>[4x]MNNTHGVDSRSDRTSPQDLASAEVAGLPVSALHGTNISTGRGSEADVAEPIQEAVDRKVSELDLAAYDKDDFTQPMIKKIMSRLFSAFDVTHLGYLTPDKVEEVCRYLGRNMSDGDVKAMKAEINAID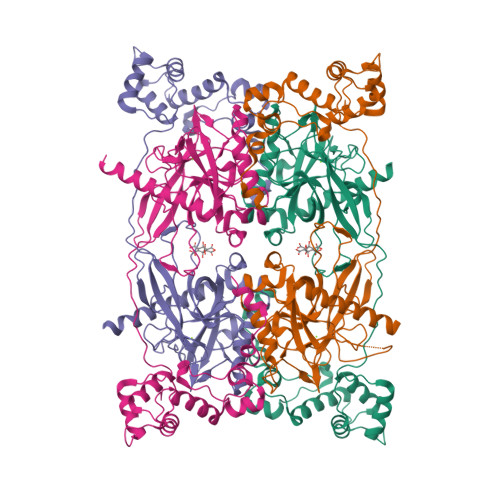GHVTFEKFWAWWCSHPVHSRTKCFSMVSADFSMPYHQQQLVVHEKGEMYTPSYRVLYFFRDLETGRERQVSPWHDIPLYVRDLVRTKPEATPMNRYNFICEIPKWTRAKFEIATGESFNPIKQDIKNGVPRFYKHGDMMWNYGAFPQTWESTEVLFEAGVTGDNDPVDAVEIGMTQFKVGQVSAVKVLGVLGMIDEGEMDWKVVCISHSDPICHFLRDIHDVPKFLPGCLDAIREWFRVYKICQGGEASHFAFDGEFKDKEYAMKVIDESHNMWHNLRKVNKRGEL> LNPPPIAFPSFNRRCQKDWLARRAFAENEVNGRIYKNVYQNLGFKGPIPILNKVGQYRIRMRCISGGYSRGIFRFTRMARMGMLQLAREGWLKKY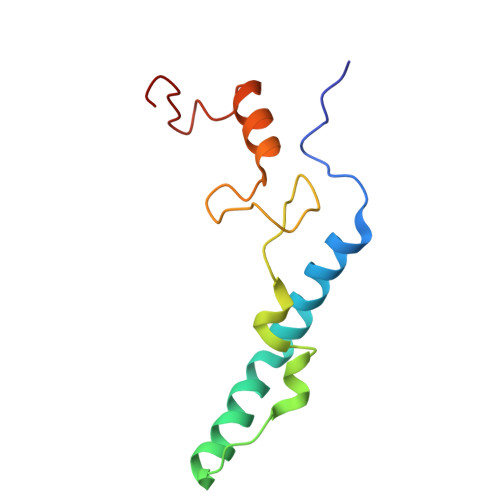GYRPGLF>GSHMAITKINDCFELLSMVTYADKLKSLIKKEFSISFEEFAVLTYISENKEKEYYLKDIINHLNYKQPQVVK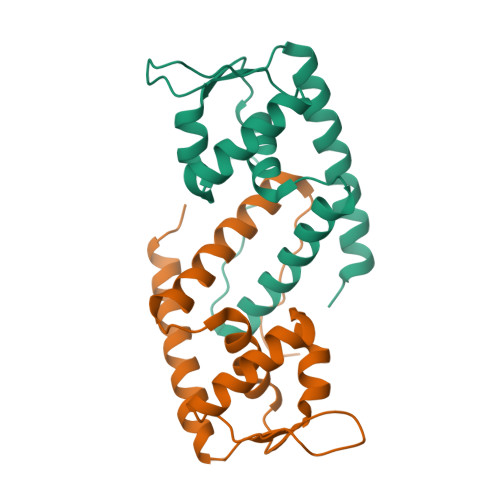AVKILSQEDYFDKKRNEHDERTVLILVNAQQRKKIESLLSRVNKRITEANNEIEL[2x]>[4x]MAREPTALATAAAIRSGATTARAETEAAIARIEALDGAIN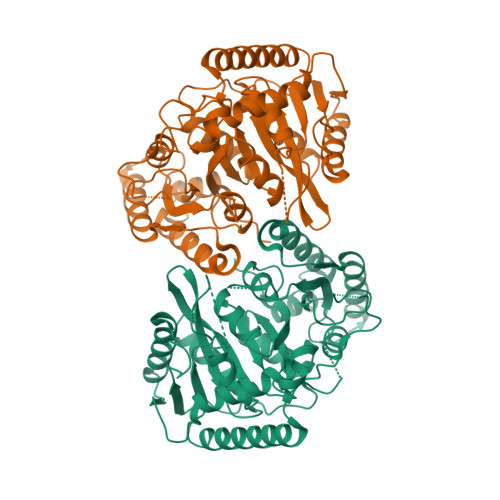AVVVRDFDRALAAADAADARIQAGDTAPLLGVPMTVKEAFDVEGLPTHWGFRQHAGNIATSDAEAVRRLKAAGAIILGKTNVPKGLGDWQSVNSIHGVTNHPLDPTRTPGGSSGGSAAALASGMVPLELGSDIGGSIRIPAHFCGVWGLKPSWGAISSHGHRYPGTNGAETPLGVIGPMARSPDDLAAMLDLLATLPMPRASRPPRRVLAITDHPAIRTSAVCRDAVDTAAEALAGAGIEVIRSTDLLPDLARQHHAYGQMLSVAFARSDPTLHASLPNLLTWLSWQDAQARNTRAWGRLFGEVDAVIAPPAATQAFAHDHAPQANRTLDIDGVASPYDAHLAWAGVATYPGLPAVVVPVGTANGLPVGVQVITDFHRDHDAIATAALIHRLTEGQPALEHHHHHH> NESGNEGVIINNFYSNQYQNSIDLSASGGNAGD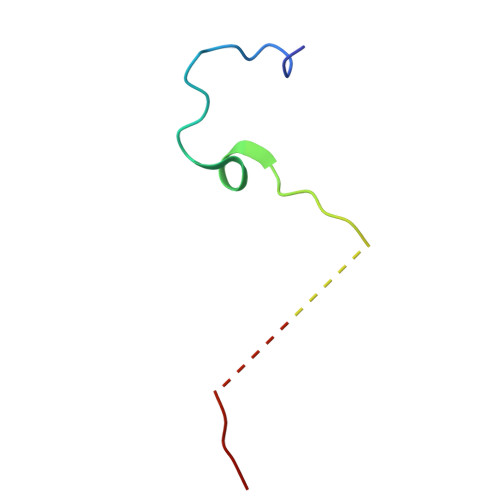APQTNGQLSNLL> SYVMPQSFAFVFPGQGSQHLGMLAELGLQQPIVLETFQQASSALAYDLWALVQHGPQERLDQTQFTQPALLTADVAIFRCWEALGGPKPQVMAGHSLGEYAALVCAGALKFEEAVKLVEKRGQYMQEAVPVGEGAMGAIIGLNEAEIESICENAALGQVVQPANLNSTDQTVISGHSEAVDRALNMAKTEGAKIAKRIPVSVPSHCPLMQPAADRLAQDIAKISIDSPKVPVIHNVDVVDHNEANIIRGALIKQLVRPVRWVETIKYIEEQGIKVFMECGPDNKLAGLIKRIDRQSEILPLTTTELILT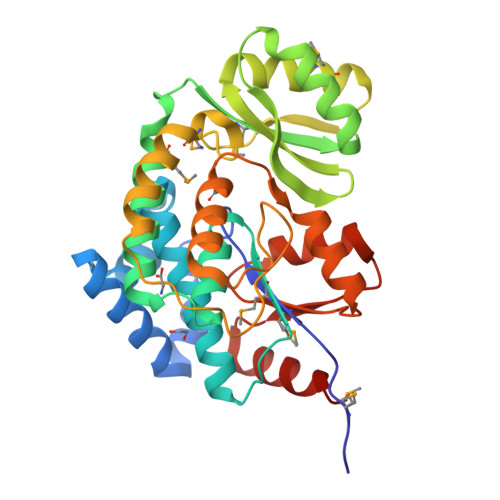AIKRLTH(7R)-8-(cyclopropylmethyl)-2-[(3,5-difluoro-4-hydroxyphenyl)amino]-7-methyl-5-(prop-2-yn-1-yl)-7,8-dihydropteridin-6(5H)-one | 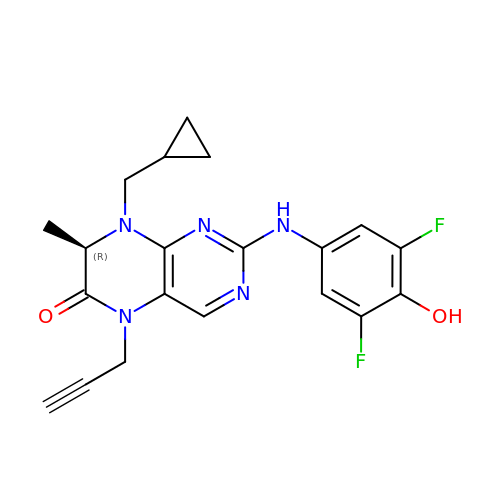C20 H19 F2 N5 O2 | VCABIQKTZQAYKL-LLVKDONJSA-N> MGHHHH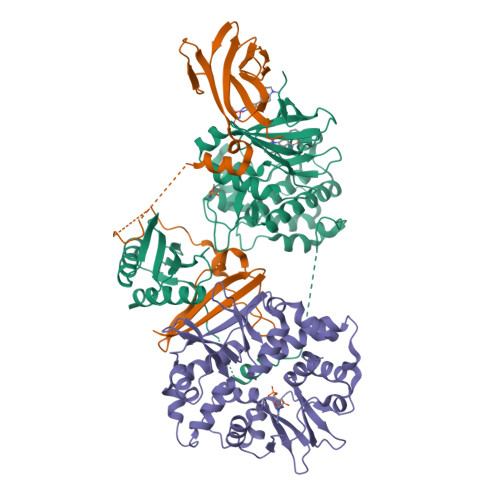HHGSVKIGHYILGDTLGVGTFGKVKVGKHELTGHKVAVKILNRQKIRSLDVVGKIRREIQNLKLFRHPHIIKLYQVISTPSDIFMVMEYVSGGELFDYICKNGRLDEKESRRLFQQILSGVDYCHRHMVVHRDLKPENVLLDAHMNAKIADFGLSNMMSDGEFLRTSCGSPNYAAPEVISGRLYAGPEVDIWSSGVILYALLCGTLPFDDDHVPTLFKKICDGIFYTPQYLNPSVISLLKHMLQVDPMKRATIKDIREHEWFKQDLPKYLFPEDPSYSSTMIDDEALKEVCEKFECSEEEVLSCLYNRNHQDPLAVAYHLIIDNRRIMNEAKDFYLATSPPDSFLDDHHLTRPHPERVPFLVAETPRARHTLDELNPQKSKHQGVRKAKWHLGIRSQSRPNDIMAEVCRAIKQLDYEWKVVNPYYLRVRRKNPVTSTYSKMSLQLYQVDSRTYLLDFRSIDDELTPRPGSHTIEFFEMCANLIKILAQ;> MEVNDKAPAQARPTVFRWTGGGKEVYLSGSFNNWSKLPLTRDHNNFVAILDLPEGEHQYKFFVDGQWTHDPSEPIVTSQLGTVNNIIQVKKTDFEVFDALMVDSQKCSDVSELSSSPPGPYHQEPYVCKPEERFRAPPILPPHLLQVILNKDTGISCDPALLPEPNHVMLNHLYALSIKDGVMVLSATHRYKKKYVTTLLYKPI;> METVISSDSSPAVENEHPQETPESNNSVYTSFMKSHRCYDLIPTSSKLVVFDTSLQVKKAFFALVTNGVRAAPLWDSKKQSFVGMLTITDFINILHRYYKSALVQIYELEEHKIETWREVYLQDSFKPLVCISPNASLFDAVSSLIRNKIHRLPVIDPESGNTLYILTHKRILKFLKLFITEFPKPEFMSKSLEELQIGTYANIAMVRTTTPVYVALGIFVQHRVSALPVVDEKGRVVDIYSKFDVINLAAEKTYNNLDVSVTKALQHRSHYFEGVLKCYLHETLETIINRLVEAEVHRLVVVDENDVVKGIVSLSDILQALVLT>[2x]MPTPSMEDYLE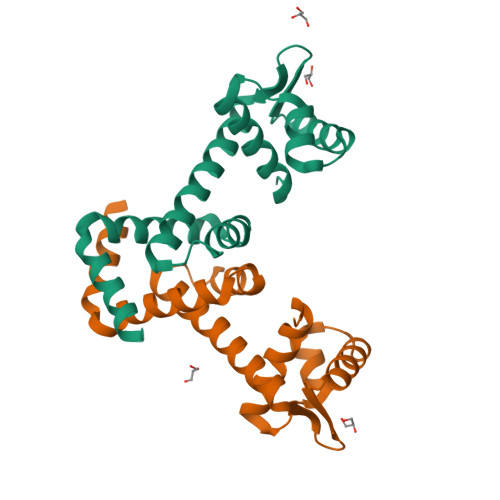RIYLLIEEKGYARVSDIAEALEVHPSSVTKMVQKLDKSDYLVYERYRGLILTAKGKKIGKRLVYRHDLLEDFLKMIGVDSDHIYEDVEGIEHHLSWDAIDRIGDLVQYFQEDPSRLNDLREVQKKNEE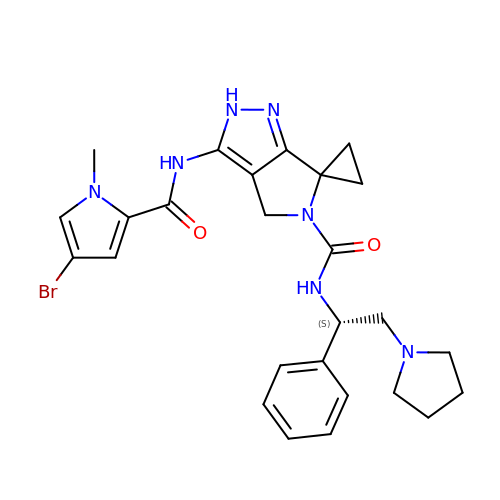3'-{[(4-bromo-1-methyl-1H-pyrrol-2-yl)carbonyl]amino}-N-[(1S)-1-phenyl-2-(pyrrolidin-1-yl)ethyl]-1',4'-dihydro-5'H-spiro[cyclopropane-1,6'-pyrrolo[3,4-c]pyrazole]-5'-carboxamide | C26 H30 Br N7 O2 | FWWFONGGISSNJV-HXUWFJFHSA-N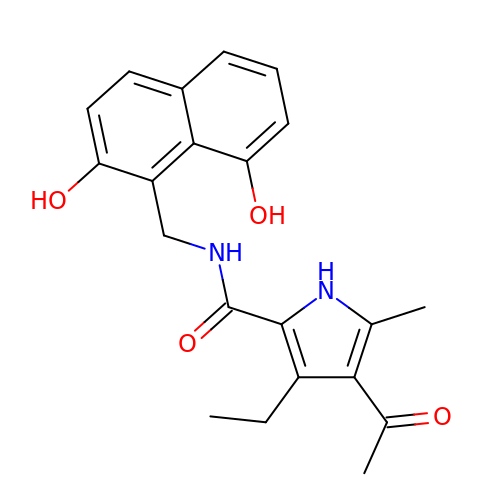~{N}-[[2,8-bis(oxidanyl)naphthalen-1-yl]methyl]-4-ethanoyl-3-ethyl-5-methyl-1~{H}-pyrrole-2-carboxamide | C21 H22 N2 O4 | KCGVENSOXCWCNF-UHFFFAOYSA-N>[2x]MSLAKNIVFIGESGSGKSTLARALAKDLDLVFLDSDFLIEQKFNQKASEIWE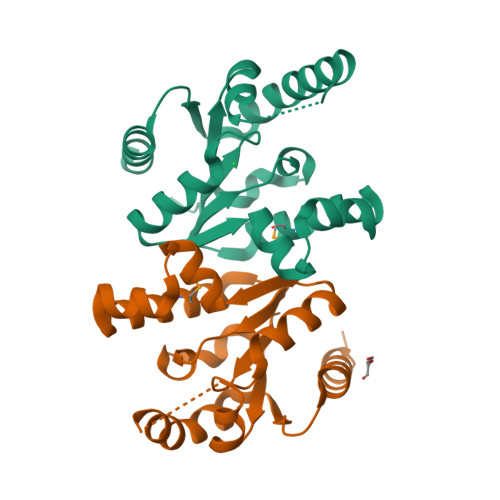QYGWNFALEQEQKMADFFSSCEKACIATSGSFVNVSNLEKAGFCIYLKADFEYLKKRLDKDEISKFPLFSDEIKWKKHYNETLSKYEQKANFILNIENKNIDELLSEIKKVIKLEHHHHHH> MEIKRFGRIREVIPLPPLTEIQVESYKKALQADVPPEKRENVGIQAAFKETFPIEEGDKGKGGLVLDFLEYRIGDPPFSQDECREKDLTYQAPLYARLQLIHKDTGLIKEDEVFLGHLPLMTEDGSFIINGADRVIVSQIHRSPGVYFTPDPARPGRYIASIIPLPKRGPWIDLEVEASGVVTMKVNKRKFPLVLLLRVLGYDQETLVRELSAYGDLVQGLLDEAVLAMRPEEAMVRLFTLLRPGDPPKKDKALAYLFGLLADPKRYDLGEAGRYKAEEKLGVGLSGRTLVRFEDGEFKDEVFLPTLRYLFALTAGVPGHEVDDIDHLGNRRIRTVGELMADQFRVGLARLARGVRERMVMGSPDTLTPAKLVNSRPLEAALREFFSRSQLSQFKDETNPLSSLRHKRRISALGPGGLTRERAGFDVRDVHRTHYGRICPVETPEGANIGLITSLAAYARVDALGFIRTPYRRVKNGVVTEEVVYMTASEEDRYTIAQANTPLEGDRIATDRVVARRRGEPVIVAPEEVEFMDVSPKQVFSLNTNLIPFLEHDDANRALMGSNMQTQAVPLIRAQAPVVMTGLEERVVRDSLAALYAEEDGEVVKVDGTRIAVRYEDGRLVEHPLRRYARSNQGTAFDQRPRVRVGQRVKKGDLLADGPASEEGFLALGQNVLVAIMPFDGYNFEDAIVISEELLKRDFYTSIHIERYEIEARDTKLGPERITRDIPHLSEAALRDLDEEGIVRIGAEVKPGDILVGRTSFKGEQEPSPEERLLRSIFGEKARDVKDTSLRVPPGEGGIVVGRLRLRRGDPGVELKPGVREVVRVFVAQKRKLQVGDKLANRHGNKGVVAKILPVEDMPHLPDGTPVDVILNPLGVPSRMNLGQILETHLGLAGYFLGQRYISPVFDGATEPEIKELLAEAFNLYFGKRQGEGFGVDKREKEVLARAEKLGLVSPGKSPEEQLKELFDLGKVVLYDGRTGEPFEG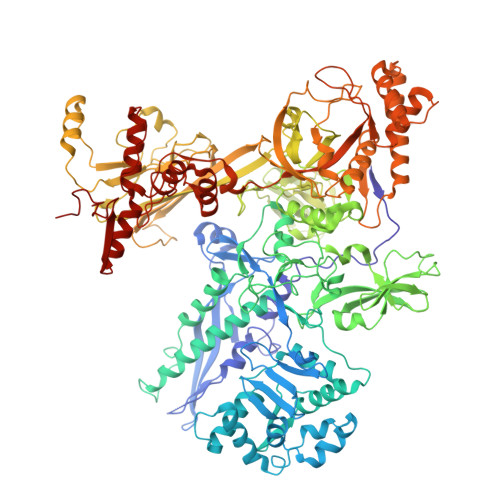PIVVGQMFIMKLYHMVEDKMHARSTGPYSLITQQPLGGKAQFGGQRFGEMEVWALEAYGAAHTLQEMLTIKSDDIEGRNAAYQAIIKGEDVPEPSVPESFRVLVKELQALALDVQTLDEKDNPVDIFEGLASKR> VGLTTLFWLGAIGMLVGTLAFAWAGRDAGSGERRYYVTLVGISGIAAVAYVVMALGVGWVPVAERTVFAPRYIDWILTTPLIVYFLGLLAGLDSREFGIVITLNTVVMLAGFAGAMVPGIERYALFGMGAVAFLGLVYYLVGPMTESASQRSSGIKSLYVRLRNLTVILWAIYPFIWLLGPPGVALLTPTVDVALIVYLDLVTKVGFGFIALDAAATLRAEHGESLAGVDTDAPAVADENSHHHHHHH;> AVSRLLLPSRVRHSYTGKMGAVFIFVGALTVLFGAIAYGEVTAAAATGDAAAVQEAAVSAILGLIILLGINLGLVAATLGGDTAASLSTLAAKASRMGDGDLDVELETRREDEIGDL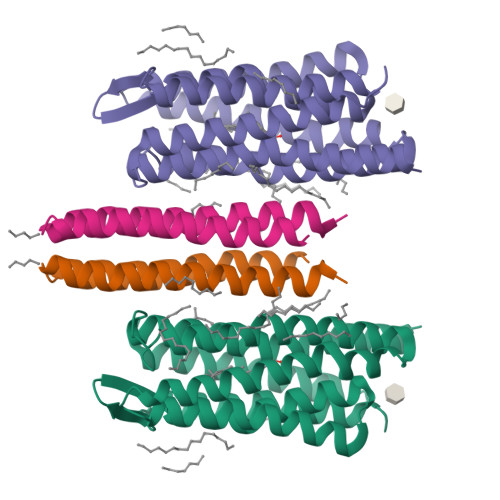YAAFDEMRQSVRTSLEDAKNAREDAEQAQKRAEEINTNSHHHHHHH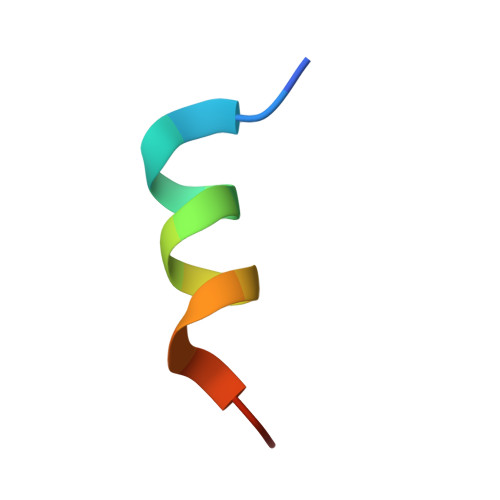> KETAAAKFERQHVDSX>[2x]LSE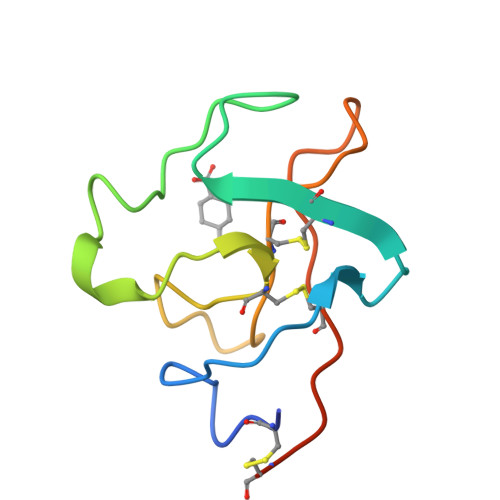CKTGNGKNYRGTMSKTKNGITCQKWSSTSPHRPRFSPATHPSEGLEENYCRNPDNDPQGPWCYTTDPEKRYDYCDILECEEECMH> EPPTACREKQYLINSQCCSLCQPGQKLVSDCTEFTETECLPCGESEFLDTWNRETHCHQHKYCDPNLGLRVQQKGTSETDTICTCEEGWHCTSEACESCVLHRSCSP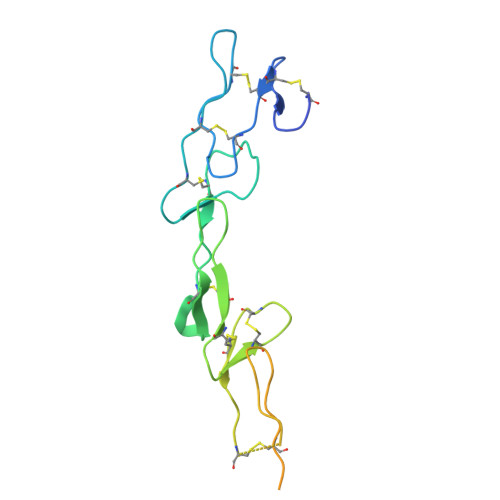GFGVKQIATGVSDTICEPCPVGFFSNVSSAFEKCHPWTSCETKDLVVQQAGTNKTDVVCGPQDSGRLVPR> GKNPVESVSVEFEAKSARDGAWYDVAAFLSHRLFESGDPEVRVRFSGFGAEEDEWINVRKCVRQRSLPCEATECVAVLPGDLILCFQEGKDQALYYDAHVLDAQRRRHDVGGCRCRFLVRYDHDSSEEIVPLRKVCRRP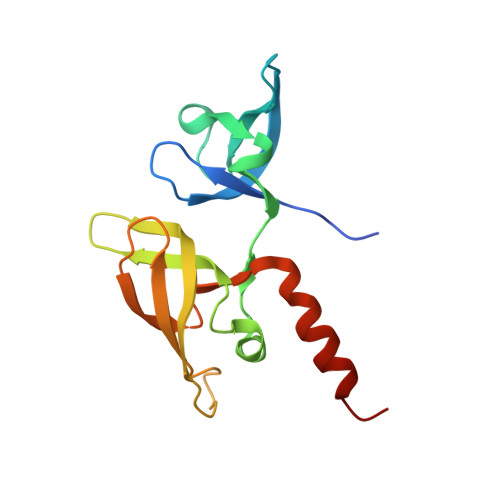ETDYRLQILHAARAAATN>[2x]MPSSHPHITHRYRVPSSDDHERISALFLGPKAENAAFLQQWLTTVVAQQKAARDAYFPDDNAFITTDMQTSPAFAQTTKVIASNLTELLTALGERSIPFFSPRYSGHMSVDQSLPAILGFLSTTFYNPNNVAFEASPFTTLIEEEVGLQLSEMLGYNRLNNTEKPLAWGHIASGGTVANLEAMWAARNLKFYPLSLRDASAEGAEMEFIRDTFSVKTCVGDKKLLKDCSPWELLNLHVSTILDMPDRLHDEYNISPQFLEKVMRKYIIQSTNKDTLMQRWGLTQQPVVLS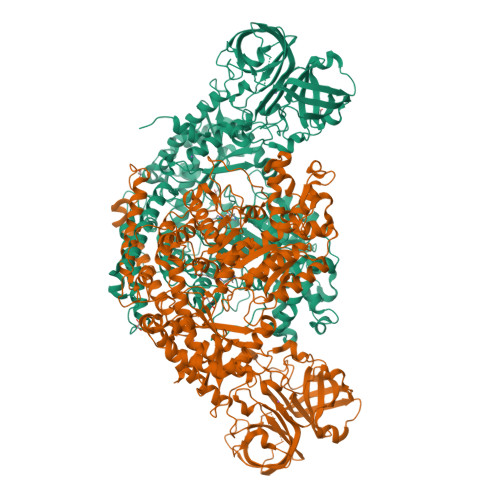PSTNHYSWPKAAAVLGIGSDNLRNVPVDIQAHMDINELDRMLKICLDEETPVYQVVAVIGTTEEGGVDRITEILKLRQKYEALGLSFAIHADAAWGGYFATMLPKDTLGRNRTRLPKEDTTSGFVPHVGLREESALQLSHIKYADSITIDPHKAGYVPYPAGALCYRDGRMRYLLTWSAPYLAQGNEGQSIGIYGIEGSKPGAAASAVFMAHETIGLTPSGYGNLLGQAMFTCRRYAAHWSAMSTDTTSFTVTPFNPIPADIDPNADPAKVEEQKQFIRDRILFKSNEEIYNDSEAMELLHQLGSDLNINVFACNFRDRDNNLNTDVEEANWLNNRIFQRFSVTSAEENPLETPFFLSSTTLKQSEYGVCATEVKRRMGLVGDQDVIVLRNVVMSPFTTTNDFVGTLANTFQKIVEEEVEYARIRNDMKPSIHTFLLHGSGEQYYLVHTPTIHMASGRRQIILSVNVEGQVRQAIHAHERVEAVIVHNTVPLRLDEIVDGGSFDGILTIGKRKTSFKVKISNIKVVKKRSLMTEDLESAYPSLMPFYFYGTQGHAHLDHVITVVPNIHLSAGEIQYKFDDEVSSEDLAKGLIVVAENVHEASMQPFPLMKDFKITNQFFFSSGQILRVKVYRDPYPASTMDPIPLHDIKNQPVVTQGTITLVGNIYVDSDALNVASEPTADEDAAHVPHARNMYGEMTAGTIKGWQNAVRHFHNKLETVAPTK> SINGGIRAATSQEINELTYYTTLSANSYCRTVIPGATWDCIHCDATEDLKIIKTWSTLIYDTNAMVARGDSEKTIYIVFRGSSSIRNWIADLTFVPVSYPPVSGTKVHKGFL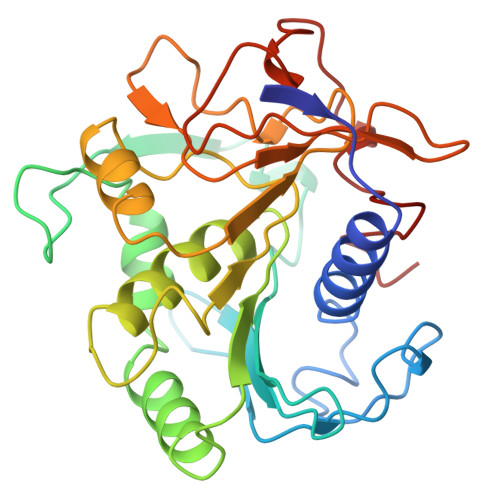DSYGEVQNELVATVLDQFKQYPSYKVAVTGHSLGGATALLCALDLYQREEGLSSSNLFLYTQGQPRVGNPAFANYVVSTGIPYRRTVNERDIVPHLPPAAFGFLHAGSEYWITDNSPETVQVCTSDLETSDCSNSIVPFTSVLDHLSYFGINTGLCS> SIWDIEKASLLVNDCQNIANMAEQKVMMVSAIFSESSKDIVNPESFSERLGKETVKDLYEFNEQLTTKYGLEFRTIFFSYIRKYDAYWCLFEDLEKPLKSIQFFTGLIDLLDNTNKHLTLRSIVLDALLSADEEDSFYGDALVLFEELVIRYFGTDSNPSIDASEF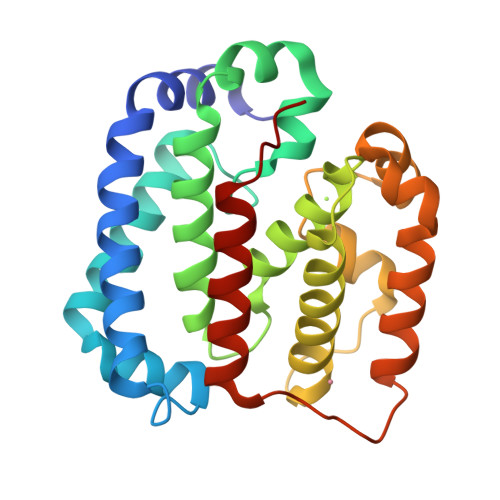ILSCLPYTSLDALNVVCGQVWKSQKICDFLKSTIGNTSNSPLQLRASFPAFVNAVIHFLLEFKNVRRLE>[4x]GSRRASVGAHMIFAVRTMVGQEKNIAGLMASRAEKEQL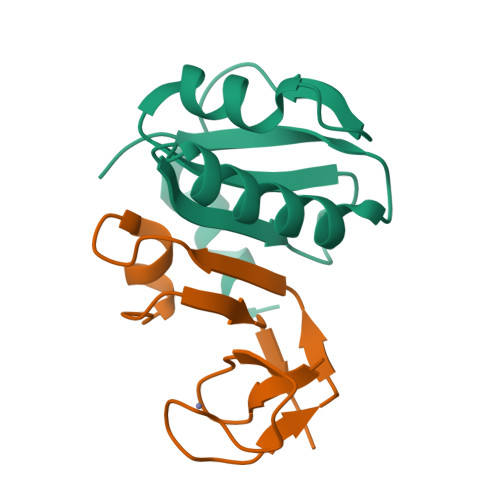DVYSILASESLKGYVLVEAETKGDVEELIKGMPRVRGIVPGTIAIEEIEPLLTP;>[4x]MRACLKCKYLTNDEICPICHSPTSENWIGLLIVINPEKSEIAKKAGIDIKGKYALSVKE>MLGTGPAAATTAATTSXXXXXXXXXXXXXXSRNEETXXXXXXXXXXXXXXXXXEMSQEEXTRFYDQLNHHIFELVSSSDANERKGGILAIASLIGVEGGNATRIGRFANYLRNLLPSNDPVVMEMASKAIGRLAMAGDTFTAEYVEFEVKRALEWLGADRNEGRRHAAVLVLRELAISVPTFFFQQVQPFFDNIFVAVWDPKQAIREGAVAALRACLILTTQREPKEMQKPQWYRHTFEEAEKGFDETLAKEKGMNRDDRIHGALLILNELVRISSMEGERLREEMEEITQQQLVHDKYCKDLMGFGTKPRHITPFTSFQAVQPQQSNALVGLLGYSSHQGLMGFGTSPSPAKSTXXXXXXXXXXXXXXXXXXXXXXXXXRNSKNSLIQMTILNLLPRLAAFRPSAFTDTQYLQDTMNHVLSCVKKEKERTAAFQALGLLSVAVRSEFKVYLPRVLDIIRAALPPKDFAHKRQKAMQVDATVFTCISMLARAMGPGIQQDIKELLEPMLAVGLSPALTAVLYDLSRQIPQLKKDIQDGLLKMLSLVLMXKPLRHPGMPKGLAHQLASPGLTTLPEASXVGSITLALRTLGSFEFEGHSLTQFVRHCADHFLNSEHKEIRMEAARTCSRLLTPSIHLISGHAHVVSQTAVQVVADVLSKLLVVGITDPDPDIRYCVLASLDERFDAHLAQAENLQALFVALNDQVFEIRELAICTVGRLSSMNPAFVMPFLRKMLIQILTELEHSGIGRIKEQSARMLGHLVSNAPRLIRPYMEPILKALILKLKDPDPDPNPGVINNVLATIGELAQVSGLEMRKWVDELFIIIMDMLQDSSLLAKRQVALWTLGQLVASTGYVVEPYRKYPTLLEVLLNFLKTEQNQGTRREAIRVLGLLGALDPYKHKVNIGMIDQSRDASAVSLSESKSSQDSSDYSTSEMLVNMGNLPLDEFYPAVSMVALMRIFRDQSLSHHHTMVVQAITFIFKSLGLKCVQFLPQVMPTFLNVIRVCDGAIREFLFQQLGMLVSFVKSHIRPYMDEIVTLMREFWVMNTSIQSTIILLIEQIVVALGGEFKLYLPQLIPHMLRVFMHDNSPGRIVSIKLLAAIQLFGANLDDYLHLLLPPIVKLFDAPEAPLPSRKAALETVDRLTESLDFTDYASRIIHPIVRTLDQSPELRSTAMDTLSSLVFQLGKKYQIFIPMVNKVLVRHRINHQRYDVLICRIVKGYTLADEEEDPLIYQHRMLRSGQGDALASGPVETGPMKKLHVSTINLQKAWGAARRVSKDDWLEWLRRLSLELLKDSSSPSLRSCWALAQAYNPMARDLFNAAFVSCWSELNEDQQDELIRSIELALTSQDIAEVTQTLLNLAEFMEHSDKGPLPLRDDNGIVLLGERAAKCRAYAKALHYKELEFQKGPTPAILESLISINNKLQQPEAAAGVLEYAMKHFGELEIQATWYEKLHEWEDALVAYDKKMDTNKDDPELMLGRMRCLEALGEWGQLHQQCCEKWTLVNDETQAKMARMAAAAAWGLGQWDSMEEYTCMIPRDTHDGAFYRAVLALHQDLFSLAQQCIDKARDLLDAELTAMAGESYSRAYGAMVSCHMLSELEEVIQYKLVPERREIIRQIWWERLQGCQRIVEDWQKILMVRSLVVSPHEDMRTWLKYASLCGKSGRLALAHKTLVLLLGVDPSRQLDHPLPTVHPQVTYAYMKNMWKSARKIDAFQHMQH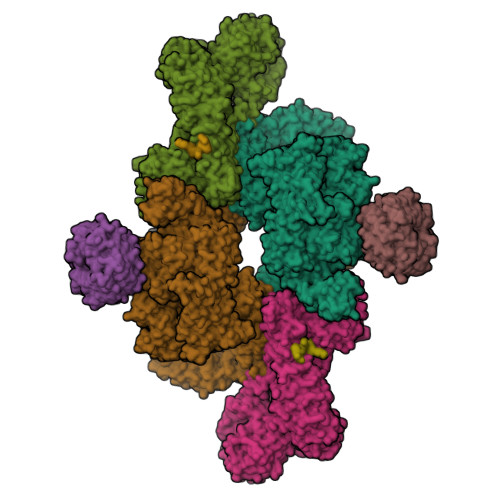FVQTMQQQAQHAIATEDQQHKQELHKLMARCFLKLGEWQLNLQGINESTIPKVLQYYSAATEHDRSWYKAWHAWAVMNFEAVLHYKHQNQARDEKKKLRHASGANITNATTAATTAATATTTASTEGSNSESEAESTENSPTPSPLQKKVTEDLSKTLLMYTVPAVQGFFRSISLSRGNNLQDTLRVLTLWFDYGHWPDVNEALVEGVKAIQIDTWLQVIPQLIARIDTPRPLVGRLIHQLLTDIGRYHPQALIYPLTVASKSTTTARHNAANKILKNMCEHSNTLVQQAMMVSEELIRVAILWHEMWHEGLEEASRLYFGERNVKGMFEVLEPLHAMMERGPQTLKETSFNQAYGRDLMEAQEWCRKYMKSGNVKDLTQAWDLYYHVFRRISKQLPQLTSLELQYVSPKLLMCRDLELAVPGTYDPNQPIIRIQSIAPSLQVITSKQRPRKLTLMGSNGHEFVFLLKGHEDLRQDERVMQLFGLVNTLLANDPTSLRKNLSIQRYAVIPLSTNSGLIGWVPHCDTLHALIRDYREKKKILLNIEHRIMLRMAPDYDHLTLMQKVEVFEHAVNNTAGDDLAKLLWLKSPSSEVWFDRRTNYTRSLAVMSMVGYILGLGDRHPSNLMLDRLSGKILHIDFGDCFEVAMTREKFPEKIPFRLTRMLTNAMEVTGLDGNYRITCHTVMEVLREHKDSVMAVLEAFVYDPLLNWRLMDTNTKGNKRSRTRTDSYSAGQSVEILDGVELGEPAHKKTGTTVPESIHSFIGDGLVKPEALNKKAIQIINRVRDKLTGRDFSHDDTLDVPTQVELLIKQATSHENLCQCYIGWCPFW[2x];>MNTSPGTVGSDPVILATAGYDHTVRFWQAHSGICTRTVQHQDSQVNALEVTPDRSMIAAAGYQHIRMYDLNSNNPNPIISYDGVNKNIASVGFHEDGRWMYTGGEDCTARIWDLRSRNLQCQRIFQVNAPINCVCLHPNQAELIVGDQSGAIHIWDLKTDHNEQLIPEPEVSITSAHIDPDASYMAAVNSTGNCYVWNLTGGIGDEVTQLIPKTKIPAHTRYALQCRFSPDSTLLATCSADQTCKIWRTSNFSLMTELSIKSGNPGESSRGWMWGCAFSGDSQYIVTASSDNLARLWCVETGEIKREYGGHQKAVVCLAFNDSVLG[2x];>GSGRMPQSKSRKIAILGYRSVGKSSLTIQFVEGQFVDSYDPTIENTFTKLITVNGQEYHLQLVDTAGQDEYSIFPQTYSIDINGYILVYSVTSIKSFEVIKVIHGKLLDMVGKVQIPIMLVGNKKDLHMERVISYEEGKALAESWNAAFLESSAKENQTAVDVFRRIILEAEKMDGAASQGKSSCSVM[2x];>MDYKDDDDKESEMLQSPLLGLGEEDEADLTDWNLPLAFMKKRHCEKIEGSKSLAQSWRMKDRMKTVSVALVLCLNVGVDPPDVVKTTPCARLECWIDPLSMGPQKALETIGANLQKQYENWQPRARYKQSLDPTVDEVKKLCTSLRRNAKEERVLFHYNGHGVPRPTVNGEVWVFNKNYTQYIPLSIYDLQTWMGSPSIFVYDCSNAGLIVKSFKQFALQREQELEVAAINPNHPLAQMPLPPSMKNCIQLAACEATELLPMIPDLPADLFTSCLTTPIKIALRWFCMQKCVSLVPGVTLDLIEKIPGRLNDRRTPLGELNWIFTAITDTIAWNVLPRDLFQKLFRQDLLVASLFRNFLLAERIMRSYNCTPVSSPRLPPTYMHAMWQAWDLAVDICLSQLPTIIEEGTAFRHSPFFAEQLTAFQVWLTMGVENRNPPEQLPIVLQVLLSQVHRLRALDLLGRFLDLGPWAVSLALSVGIFPYVLKLLQSSARELRPLLVFIWAKILAVDSSCQADLVKDNGHKYFLSVLADPYMPAEHRTMTAFILAVIVNSYHTGQEACLQGNLIAICLEQLNDPHPLLRQWVAICLGRIWQNFDSARWCGVRDSAHEKLYSLLSDPIPEVRCAAVFALGTFVGNSAERTDHSTTIDHNVAMMLAQLVSDGSPMVRKELVVALSHLVVQYESNFCTVALQFIEEEKNYALPSPATTEGGSLTPVRDSPCTPRLRSVSSYGNIRAVATARSLNKSLQNLSLTEESGGAVAFSPGNLSTSSSASSTLGSPENEEHILSFETIDKMRRASSYSSLNSLIGVSFNSVYTQIWRVLLHLAADPYPEVSDVAMKVLNSIAYKATVNARPQRVLDTSSLTQSAPASPTNKGVHIHQAGGSPPASSTSSSSLTNDVAKQPVSRDLPSGRPGTTGPAGAQYTPHSHQFPRTRKMFDKGPEQTADDADDAAGHKSFISATVQTGFCDWSARYFAQPVMKIPEEHDLESQIRKEREWRFLRNSRVRRQAQQVIQKGITRLDDQIFLNRNPGVPSVVKFHPFTPCIAVADKDSICFWDWEKGEKLDYFHNGNPRYTRVTAMEYLNGQDCSLLLTATDDGAIRVWKNFADLEKNPEMVTAWQGLSDMLPTTRGAGMVVDWEQETGLLMSSGDVRIVRIWDTDREMKVQDIPTGADSCVTSLSCDSHRSLIVAGLGDGSIRVYDRRMALSECRVMTYREHTAWVVKASLQKRPDGHIVSVSVNGDVRIFDPRMPESVNVLQIVKGLTALDIHPQADLIACGSVNQFTAIYNSSGELINNIKYYDGFMGQRVGAISCLAFHPHWPHLAVGSNDYYISVYSVEKRVR[2x];>[2x]GSGRMSGGSSCSQTPSRAIPATRRVVLGDGVQLPPGDYSTTPGGTLFSTTPGGTRIIYDRKFLMECRNSPVTKTPPRDLPTIPGVTSPSSDEPPMEASQSHLRNSPEDKRAGGEESQFEMDI>MKFGEHLSKSLIRQYSYYYISYDDLKTELEDNLSKNNGQWTQELETDFLESLEIELDKVYTFCKVKHSEVFRRVKEVQEQVQHTVRLLDSNNPPTQLDFEILEEELSDIIADVHDLAKFSRLNYTGFQKIIKKHDKKTGFILKPVFQVRLDSKPFFKENYDELVVKISQLYDIARTSGAGSDGFTVLSTKSLFLGQKLQVVQADIASIDSDAVVHPTNTDFYIGGEVGNTLEKKGGKEFVEAVLELRKKNGPLEVAGAAVSAGHGLPAKFVIHCNSPVWGADKCEELLE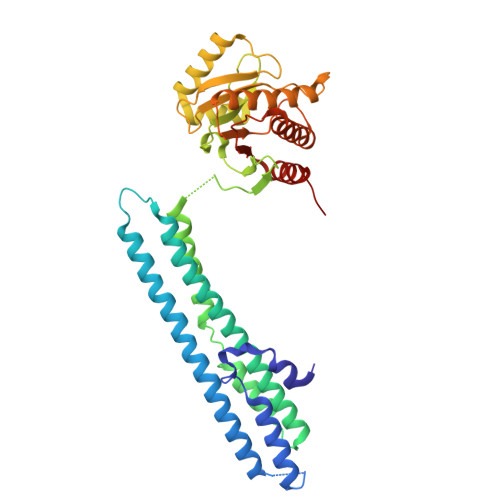KTVKNCLALADDKKLKSIAFPSIGSGRNGFPKQTAAQLILKAISSYFVSTMSSSIKTVYFVLFDSESIGIYVQEMAKLEHHHHHH[2x]Kinetoplastids (such as Trypanosoma brucei), a group of evolutionarily divergent eukaryotes, have a unique set of kinetochore proteins that lack any significant homology to canonical kinetochore components. We previously identified KKT4 as a microtubule-binding kinetochore protein in T. brucei (throughout this manuscript we refer to KKT4 from Trypanosoma brucei unless stated otherwise) (Llauro et al., 2018). KKT4 directly binds to microtubules and maintains load-bearing attachments to both growing and shortening microtubule tips in vitro. KKT4 has the following predicted regions conserved among kinetoplastid species: an N-terminal α helix, a coiled-coil region and a block of basic residues in the microtubule-binding domain, and a BRCT domain at the C terminus.

To test structural conservation in other kinetoplastid species, we attempted to solve the crystal structure of the KKT4 coiled-coil fragment from L. mexicana. We were unable to obtain diffraction-quality crystals of fragments that had the N-terminal residues of the microtubule-binding domain (115–140 in T. brucei). Instead, we crystalized and solved a 1.9 Å structure of LmKKT4184–284, which corresponds to residues 141–244 in T. brucei. We note that the expressed protein contained an additional 23 residues from the expression vector at its C terminus due to a cloning error (see the STAR Methods for details). Like TcKKT4117–218, LmKKT4184–284 has helices arranged in a parallel coiled-coil fold. LmKKT4184–284 has six regular heptad repeats from the N terminus to Q224, and after that point the helices move apart and lose their supercoiling as observed for TcKKT4117–218. The two chains in LmKKT4184–284 differ in length, with helices spanning T184 to the C terminus in one chain and T184 to R257 in the other. The region beyond I245, where the helices have moved away from each other, had high B factors in both chains, suggesting enhanced flexibility. Interestingly, the end of the longer helix, which contains extra residues from the expression vector, makes seemingly stabilizing contacts with other molecules in the crystal lattice, which potentially explains why our attempts to obtain diffraction-quality crystals for the proper construct ending at Q284 failed. Superposition of the coiled coils from T. cruzi and L. mexicana revealed a good structural match with a root-mean-square deviation (RMSD) of 1.03 Å (for 123 Cα), confirming the conservation of the coiled-coil structure in these species.

>GSTANKLTEAQRRIAELEKELQRTTQRVDQLSDVVQQQKDELQAAKDRHALEMEETRHAYNAVIHRKDEVQEEALRQLLKSRQLMVSAARYEAVVAAKKLHAQEFELGAPAGRQACGRIMLKSNRK[2x]>GARIKTLSVSRPIIYGNTAKKMGSVKPPNAPAEHTHLWTIFVRGPQNEDI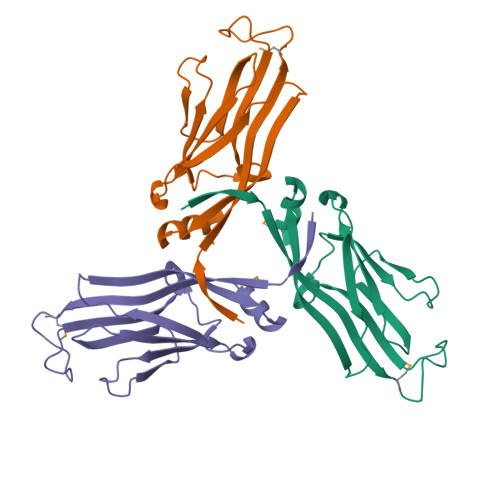SYFIKKVVFKLHDTYPNPVRSIEAPPFELTETGWGEFDINIKVYFVEEANEKVLNFYHRLRLHPYANPVPNSDNGNEQNTTDHNSKDAEVSSVYFDEIVFNEPNEEFFKILMSR[3x]> GMPKPINVRVTTMDAELEFAIQPNTTGKQLFDQVVKTIGLREVWYFGLHYVDNKGFPTWLKLDKKVSAQEVRKENPLQFKFRAKFYPEDVAEELIQDIT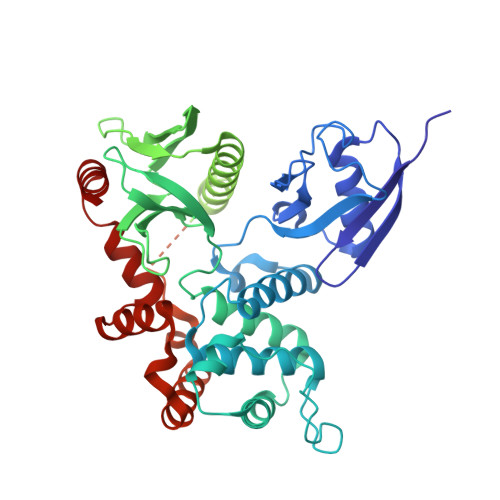QKLFFLQVKEGILSDEIYCPPETAVLLGSYAVQAKFGDYNKEVHKSGYLSSERLIPQRVMDQHKLTRDQWEDRIQVWHAEHRGMLKDNAMLEYLKIAQDLEMYGINYFEIKNKKGTDLWLGVDALGLNIYEKDDKLTPKIGFPWSEIRNISFNDKKFVIKPIDKKAPDFVFYAPRLRINKRILQLCMGNHELYMRRRKPDTIEVQQMKAQAREEKHQKQLERQQLETEKKRRETVEREKEQMMREKEELMLRLQDYEEKTKKAERELSEQIQRALQLEEERKRAQEEAERLEADRMAALRAKEELERQAVDQIKSQEQLAAELAEYTAKIALLEEARRRKEDEVEEWQHRAKEAQDDLVKTKEELHLVMTAPPPPPPPVYEPVSYHVQESLQDEGAEPTGYSAELSSEGIRDDRNEEKRITEAEKNERVQRQLLTLSSELSQARDENKRTHNDIIHNENMRQGRDKYKTLRQIRQGNTKQRIDEFEAL>[6x]GSRARRPHNAIFVNFEDEEVPKQPLEAAAQTWRRVCTNPVDRKVEEELRKLFDIRPIWSRNAVKANISVHP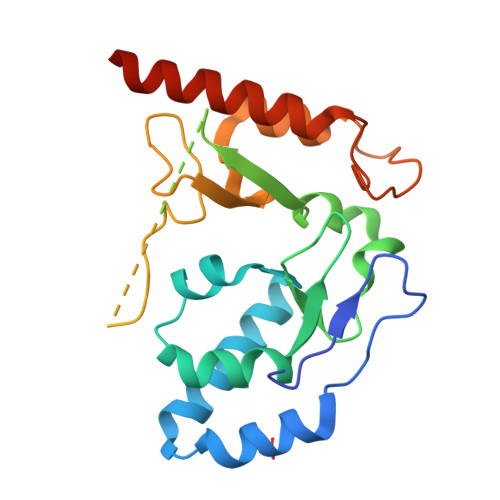DKLKVLLPFIAYYMITGPWRSLWIRFGYDPRKNPDAKIYQVLDFRIRCGMKHGYAPSDLPVKAKRSTKQGLGPSGTSGARKPASSKYKLKDSVYIFREGALPPYRQMFYQLCDLNVEELQKIIHRNDGAENSCTERDGWCLPKTSDELRDTMSLMIRQTIRSKRPALFSSS>[2x]AHMMEKLKEIEKVTKAIKEKILNHYGYIRVITHHDTDGLSSGGILAKMLMRTNKLFHLTVVEHLSKEVIEKLAKENEVNKPLFIFAAMGSGQIEEIIKHNFNAIILDHHPPVIKDSFINENI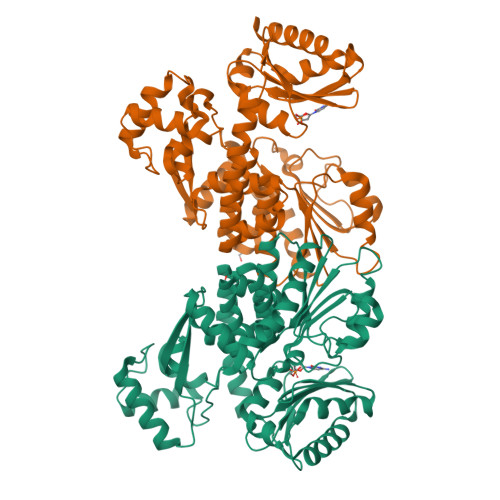IQLNPHIFGVDGSREITASGVCYLVAREFGYYDLSVLAIVGIIGDMQYNPLLGLNKFIVNEAREYRYVKIMNDIVYNIYDVEIYKAIAYCTKPYIPDLASEGKAFKFLKDIGIDPNKKQLDDTDKKKLLSAIIFKYPKIENLLIDRYLIEHKVRDAFLLSEMLNAVGRNGLFAVGIGICLEDDECIKIGNQILWEYKKNLINELKSVKLKKLNNIYYFEGKKGMIGIIASILVDDKPVIGYHIEGDIAKFSARGNRDLVNRGLNLSVAMAVAKEFGGNGGGHDVASGAVVSKDKVQEFLKRVDEIIGEQLRR>[2x]LRQCLP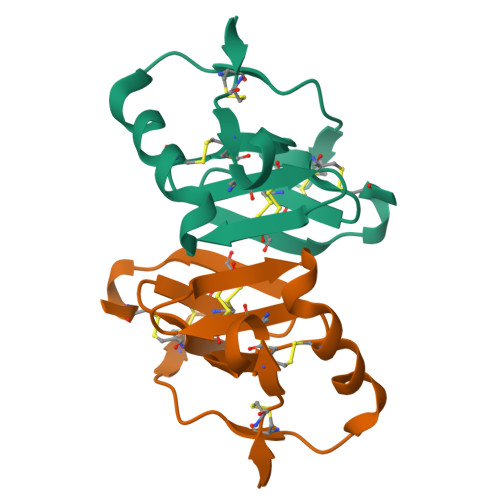CGPGGKGRCFGPSICCGDELGCFVGTAEALRCQEENYLPSPCQSGQKPCGSGGRCAAAGICCNDESCVTEPECREGVGFPRRV> MNSPF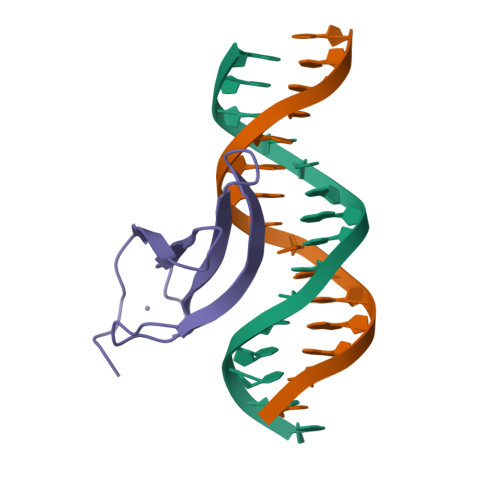IREKVMEDGYNWRKYGQKLVKGNEFVRSYYRCTHPNCKAKKQLERSAGGQVVDTVYFGEHDHPKPLCLEHHHHHH> GSMVEATAQETDRPRFSFSIAAREGKARTGTIEMKRGVIRTPAFMPVGTAATVKALKPETVRATGADIILGNTYHLMLRPGAERIAKLGGLHSFMGWDRPILTDSGGYQVMSLSSLTKQSEEGVTFKSHLDGSRHMLSPERSIEIQHLLGSDIVMAFDECTPYPATPSRAASSMERSMRWAKRSRDAFDSRKEQAENAALFGIQQGSVFENLRQQSADALAEIGFDGYAVGGLAVGEGQDEMFRVLDFSVPMLPDDKPHYLMGCGKPDDIVGAVERGIDMFDCVLP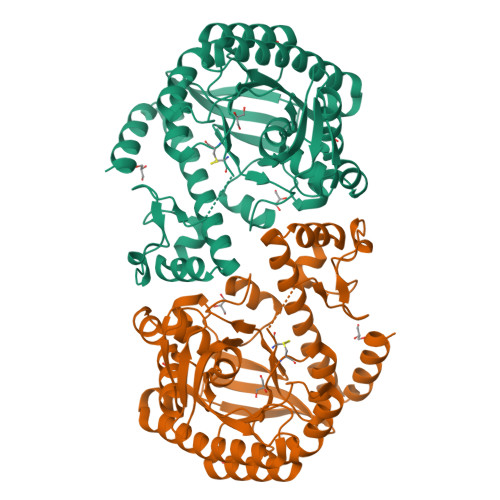TRSGRNGQAFTWDGPINIRNARFSEDLKPLDSECHCAVCQKWSRAYIHHLIRAGEILGAMLMTEHNIAFYQQLMQKIRDSISEGRFSQFAQDFRARYFARNS>GPGSMMVLDIQLFRDETGANIIRESQRRRFADPDIVDAIIEADKKWRRTQFLTEASKKLINICSKAVGAKKKAKEADGDTSEIPPQVKEAYENGTLKGEQVEQLCVLQLKQLSKDLSDQVAGLAKEAQQLEEERDKLMLNVGNILHESVPIAQDEETGNTVVRTFGNTTKRAKLNHVSIMERLGMMDTSKAVTSMAGGRSYVLKGGLVQLQVALVSYSLDFLVKRGYTPFYPPFFLNRDVMGEVAQLSQFDEELYQVSGDGDKKYLIATSEMPIAAYHRGRWFTELKEPLKYAGMSTCF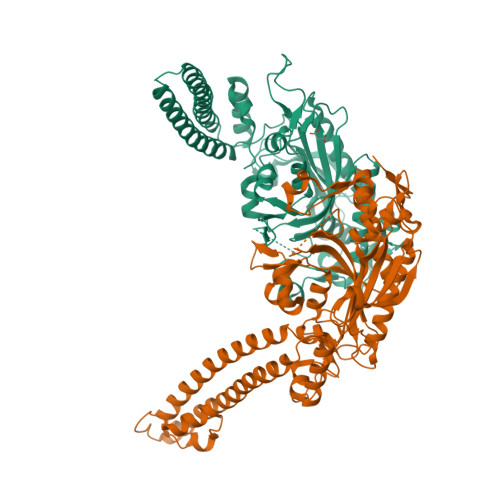RKEAGAHGRDTLGIFRVHQFDKIEQFVVCSPRQEESWRHLEDMITTSEEFNKSLGLPYRVVNICSGALNNAAAKKYDLEAWFPASGAFRELVSCSNCTDYQSQSVNCRYGPNLRGTAAQNVKEYCHMLNGTLCAITRTMCCICENYQTEEGVVIPDVLRPYMMGIEMIRFENNAQAEGTTPDKGE[2x]>MSYNNPNNSNSHLRPHAYNNSRRDDSDGDESSIEFLNQRSNTPLTQGTYNYHNTSTNSLNFQQPEPIYRNQTRTSLSDSYYDHPIFDTSQTQIQPPHDNPFTESYEMTDTSYQGNDHHYRTGQPNHLMNPTYNQAFIPHVYDEEDNDEQEYDQRIQYNQFQGDHFDLAAISYADDESQSQLDYVPTERVIPEGEEEEEEGETSFEKEPGSETISGPFGEERSFEEPPPQQEVRSKKLTRATGLNGHLVLDCPVADELLSKFPDYNPAEKSGGLSREFAFMRYTAVTCGPSNFYRDAYILRPVHYPIPRQTELMIVITMYNEDDILLGRTLKGVFKNIKYLESKARSSTWGKDSWKKIVVCIVSDGRTKINERAQALLAGLGVYQEGLAKSRVDDKKVQAHMFEYTTRVGISKVTDDVVKLTTEKVVPVQMLFCLKETNAKKINSHRWCFQAIGQVLDPKIVVLLDCGTQPSGRSLYELWKEFDRDHRVAGACGEITTSLKK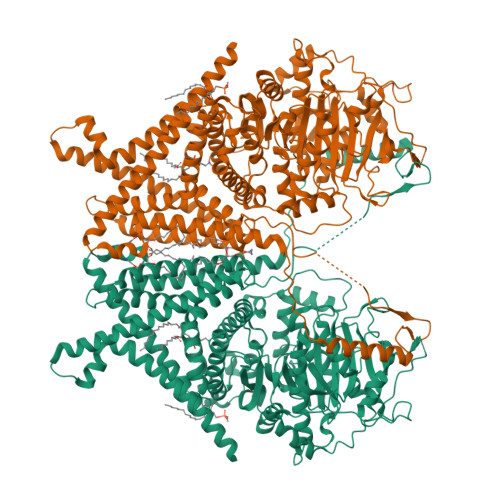RQMITNPLVYGQNFEYKISNILDKPTESSFGFISVLPGAFSAYRFIALQNDINGVGPLEKYFKGEFLHSSGELDPNDDEFQMKHLMLKEEAGIFTSNMYLAEDRILCFELVAKRGCNWLLRYCKSARAETDVPEGLAEFILQRRRWLNGSFFAAIYSLVHFYKVWTSSHSFGRKIFLHIEFFYQLINLIVSWFSIGSYFLVFRILTTSLGDKALGFAPGKILSVIFLWLYLASIVTTFVLSFGNKPKGTEKFYVTIVIFFAILMAYMIFAAIFMAVHSIQDIYRSGTRITVSLFFQNSEFRDLVVATSSTYALYFLASFLYFEPWHMFTSFVQYILLSPSYVNVLNIYAFCNIDDISWGTKGEVGGKSLGEAKLREDGTFDVSVPISKEQINQSYLDQLEKIRDPAPPEEKVLVTNTEDYYAFIRSMTVLVWMFTNFVVIALVLETGGFNQFVEATDLANLKSNRAAVFLTVILWTVAFMALFRFIGCIYYLITRLGREIKASEHATKANSLEVLFQGPDYKDDDDKAHHHHHHHHHH[2x]>ITSSKFNECQLNNLNALEPDHRVESEGGLIETWNSQHPELQCAGVTVSKRTLNRNGLHLPSYSPYPQMIIVVQGKGAIGFAFPGCPETFEKPQQQSSRRGSRSQQQLQDSHQKIRHFNEGDVLVIPPGVPYWTYNTGDEPVVAISLLDTSNFNNQLDQNPRVFYLAGNPDIEHPETMQQQQQQKSHGGRKQGQHQQQEEEGGSVLSGFSKHFLAQSFNTNEDTAEKLRSPDDERKQIVTVEGGLSVISPKWQEQEDEDEDEDEEYEQTPSYPPRRPSHGKHEDDEDEDEEEDQPRPDHPPQRPSRPEQQEPRGRGCQTRNGVEENICTMKLHENIARPSRADFYNPKAGRISTLNSLTLPALRQFGLSAQYVVLYRNGIYSPHWNLNANSVIYVTRGKGRVRVVNCQGNAVFDGELRRGQLLVVPQNFVVAEQGGEQGLEYVVFKTHHNAVSSYIKDVFRAIP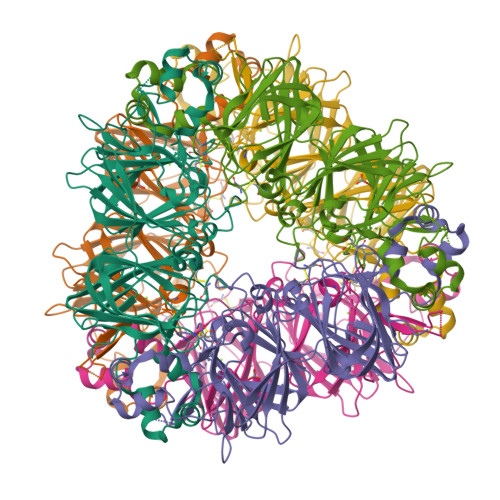SEVLSNSYNLGQSQVRQLKYQGNSGPLVNP[2x]> GLVPRGSHMIIKNYSYARQNLKALMTKVNDDSDMVTVTSTDDKNVVIMSESDYNSMMETLYLQQNPNNAEHLA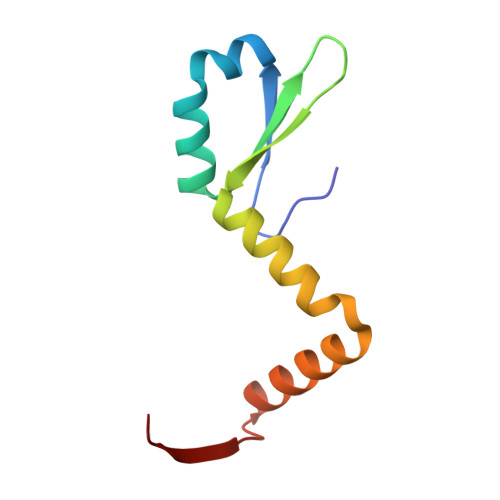QSIADLERGKTITKDIDV> GACAATTGCTGACGACACTCA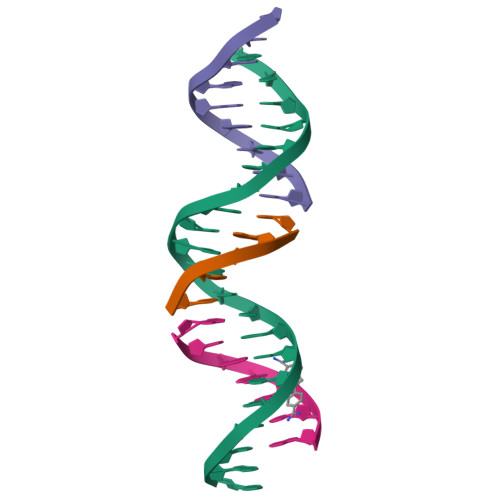;> CGTCA;> TCTGAGTGT;> GCAATTG> MASWSHPQFEKGAETAVPNSSSVPMTQNRNILWIMCDQLRFDYLSCYGHERLNTPNIDKLAKRGVRFTNAYVQATVAGPSRMSAYTGRYVRSHGSTQNGIPLRVGEPTLGDHLRDVGMRNVLIGKTHMRPDLDGMKRL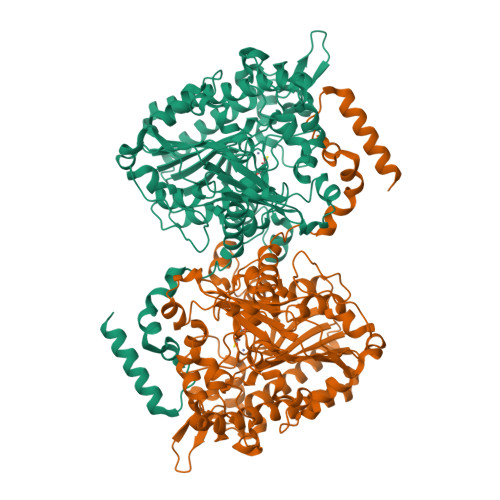GIDPDSEIGARVGEGGFDAFDRDDGVHPTGYRKKEPAYNDYLRHAGFQAENPWEFWANSAEGKGGENQSGWLLTHADKPARVPEEHSETAYMTRRAMEFMEAAEKDGRPWCAHLSYIKPHWPYIVPAPYHDMFGPDDVKPAVRSDEELKAAHPLFKAMTEEVYSRNFARDEVREKVIPAYMGLIKQIDDQLGQLFAFMQERGLDENTMIVFTADHGDYLGDHWMGEKYLFYEAAAKVPLIIYDPSDKADATRGTVSDALVEMIDLAPTFVDYAGGVPPMHILEGKSLLPLLHDDDSSWDRQYVFSELDYSNLPARLKLGRDIQDCRATMVFDGRYKLVEVMGFAPILFDLEVDPDELKDLGRDPSAEEVRQRLTSALDAWHRNTRQRITKSDAAYRALDPVLRESDPDLMAGVIIGYWDEDEVEAEKRRIARILGENS>[3x]SMTRIIGGVAGGRRIAVPPRGTRPTTDRVRESLFNIVTARRDLTGLAVLDLYAGSGALGLEALSRGAASVLFVESDQRSAA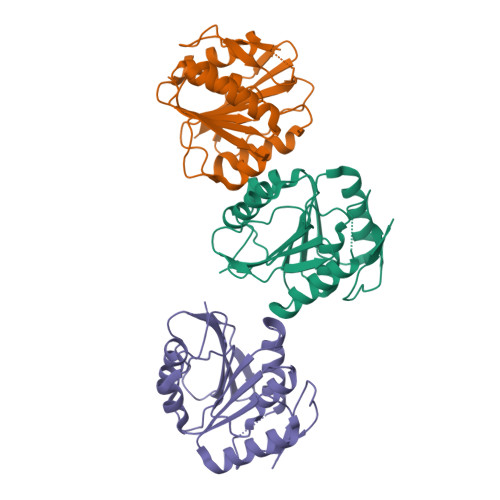VIARNIEALGLSGATLRRGAVAAVVAAGTTSPVDLVLADPPYNVDSADVDAILAALGTNGWTREGTVAVVERATTCAPLTWPEGWRRWPQRVYGDTRLELAERLFANV>[4x]GSQAPYLSPAVPF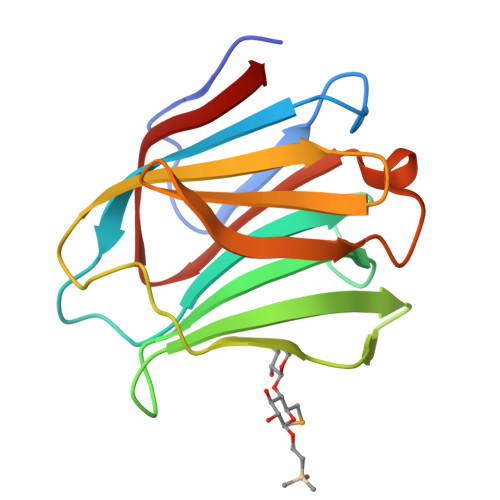SGTIQGGLQDGLQITVNGTVLSSSGTRFAVNFQTGFSGNDIAFHFNPRFEDGGYVVCNTRQNGSWGPEERKTHMPFQKGMPFDLCFLVQSSDFKVMVNGILFVQYFHRVPFHRVDTISVNGSVQLSYISFQ> MYYGISQFSEAYNKILRNSSSHSSCQLVIFVSCLNIDALCATKMLSLLFKKQLVQS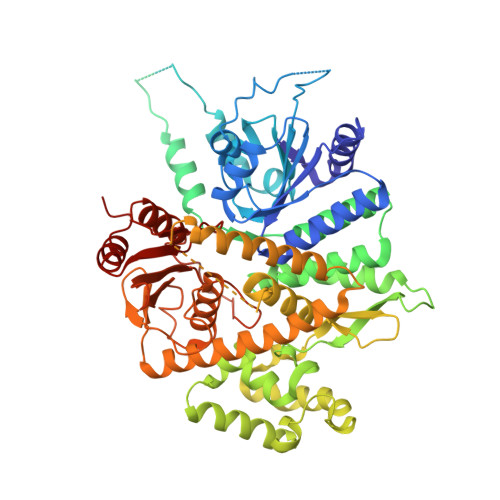QIVPIFGYSELRRHYSQLDDNINSLLLVGFGGVIDLEAFLEIDPQEYVIDTDEKSGEQSFRRDIYVLDAHRPWNLDNIFGSQIIQCFDDGTVDDTLGEQKEAYYKLLELDEESGDDELSGDENDNNGGDDEATDADEVTDEDEEDEDETISNKRGNSSIGPNDLSKRKQRKKQIHEYEGVLEEYYSQGTTVVNSISAQIYSLLSAIGETNLSNLWLNILGTTSLDIAYAQVYNRLYPLLQDEVKRLTPSSRNSVKTPDTLTLNIQPDYYLFLLRHSSLYDSFYYSNYVNAKLSLWNENGKKRLHKMFARMGIPLSTAQETWLYMDHSIKRELGIIFDKNLDRYGLQDIIRDGFVRTLGYRGSISASEFVEALTALLEVGNSTDKDSVKINNDNNDDTDGEEEEDNSAQKLTNLRKRWVSNFWLSWDALDDRKVELLNRGIQLAQDLQRAIFNTGVAILEKKLIKHLRIYRLCVLQDGPDLDLYRNPLTLLRLGNWLIECCAESEDKQLLPMVLASIDENTDTYLVAGLTPRYPRGLDTIHTKKPILNNFSMAFQQITAETDAKVRIDNFESSIIEIRREDLSPFLEKLTLSGLL>[6x]GSSCE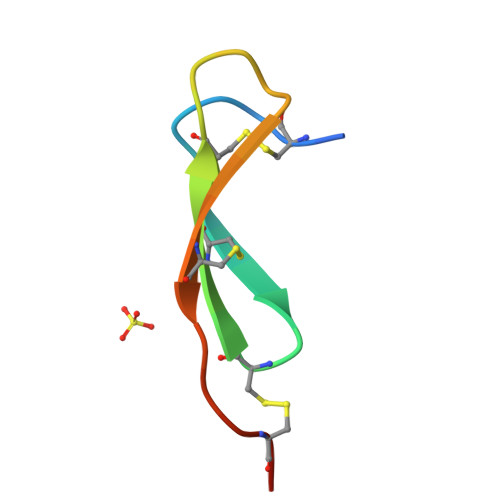PGRTFRDRCNTCKCGADGRSAACTLRACPNQ5-fluoranyl-2-methyl-benzoic 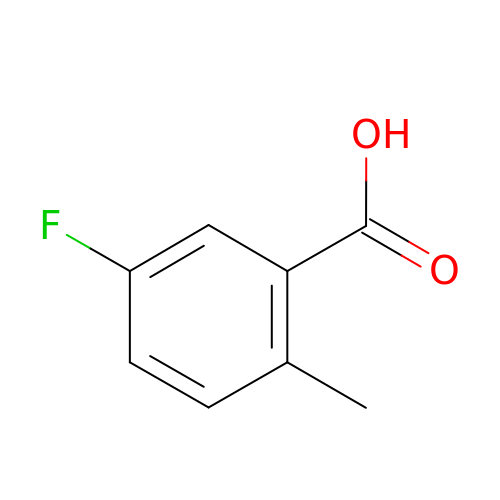acid | C8 H7 F O2 | JVBLXLBINTYFPR-UHFFFAOYSA-N>MSRLSEPSPYVEFDRRQWRALRMSTPLALTEEELVGLRGLGEQIDLLEVEEVYLPLARLIHLQVAARQRLFAATAEFLGEPQQNPDRPVPFIIGVAGSVAVGKSTTARVLQALLARWDHHPRVDLVTTDGFLYPNAELQRRNLMHRKGFPESYNRRALMRFVTSVKSGSDYACAPVYSHLHYDIIPGAEQVVRHPDILILEGLNVLQTGPTLMVSDLFDFSLYVDARIEDIEQWYVSRFLAMRTTAAA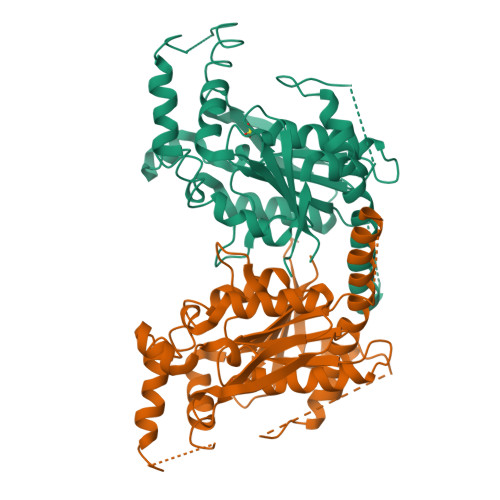DPESHFHHYAAFSDSQAVVAAREIWRTINRPNLVENILPTRPRATLVLRKDADHSINRLRLRKL[4x]(2R)-2-(3-chloro-5-fluoroanilino)-2-cyclopropyl-N-[(3R)-1-(7H-pyrrolo[2,3-d]pyrimidin-4-yl)piperidin-3-yl]acetamide | C22 H24 Cl F N6 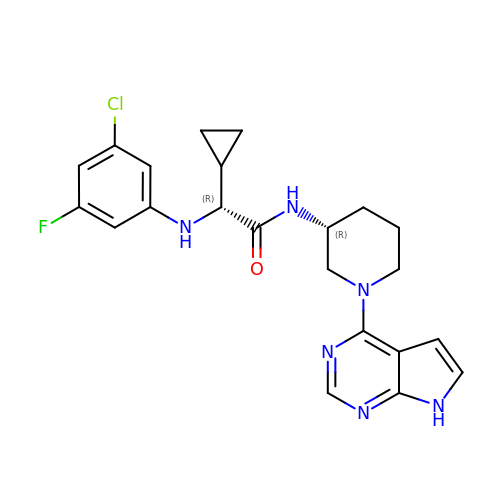O | OETOLISJTPMUFM-VQIMIIECSA-N> GPHMLEHSGISQASEYDDPPGLREKAEYLLREWVNLYHSAAAGRDSTKAFSAFVGQMHQQGILKTDDLITRFFRLCTEMCVEISYRAQAEQQHNPAANPTMIRAKCYHNLDAFVRLIALLVKHSGEATNTVTKINLLNKVLGIVVGVLLQDHDVRQSEFQQLPYHRIFIMLLLELNAPEHVLETINFQTLTAFCNTFHILRPTKAPGFVYAWLELISHRIFIARMLAHTPQQKGWPMYAQLLIDLFKYLAPFLRNVELTKPMQILYKGTLRVLLVLLHDFPEFLCDYHYGFCDVIPPNCIQLRNLILSAFPRNMRLPDPFTPNLKVDMLSEINIAPRILT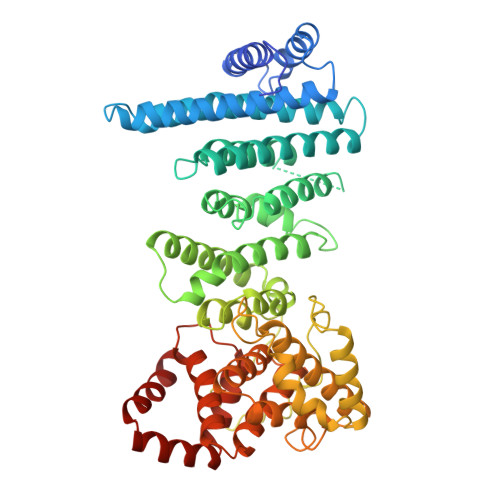NFTGVMPPQFKKDLDSYLKTRSPVTFLSDLRSNLQVSNEPGNRYNLQLINALVLYVGTQAIAHIHNKGSTPSMSTITHSAHMDIFQNLAVDLDTEGRYLFLNAIANQLRYPNSHTHYFSCTMLYLFAEANTEAIQEQITRVLLERLIVNRPHPWGLLITFIELIKNPAFKFWNHEFVEEEPEIEKLFQSVAQCCM>MTSLFTTADHYHTPLGPDGTPHAFFEALRDEAETTPIGWSEAYGGHWVVAGYKEIQAVIQNTKAFSNKGVTFPRYETGEFELMMAGQDDPVHKKYRQLVAKPFSPEATDLFTEQLRQSTNDLIDARIELGEGDAATWLANEIPARLTAILLGLPPEDGDTYRRWVWAITHVENPEEGAEIFAELVAHARTLIAERRTNPGNDIMSRVIMSKIDGESLSEDDLIGFFTILLLGGIDATARFLSSVFWRLAWDIELRRRLIAHPELIPNAVDELLRFYGPAMVGRLVTQEVT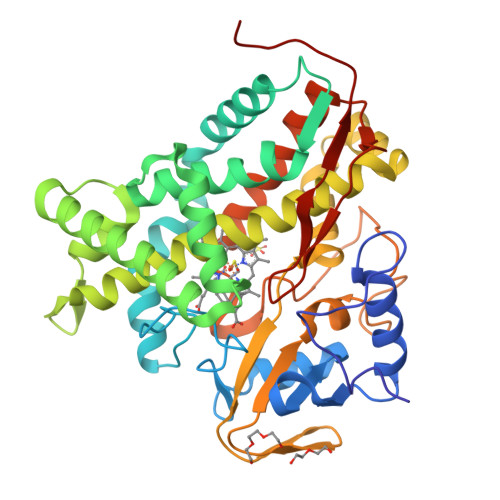VGDITMKPGQTAMLWFPIASRDRSAFDSPDNIVIERTPNRHLSLGHGIHRCLGAHLIRVEARVAITEFLKRIPEFSLDPNKECEWLMGQVAGMLHVPIIFPKGKRLSE[2x]> MSHPPSNTPPVKPGGLPLLGHILEFGKNPHAFLMALRHEFGDVAEFRMFHQRMVLLTGSQASEAFYRAPDEVLDQGPAYRIMTPIFGRGVVFDARIERKNQQLQMLMPALRDKPMRTYSEIIVAEVEAMLRDWKDAGTIDLLELTKELTIYTSSHCLLGAEFRHELNTEFAGIYRDLEMGIQPIAYVFP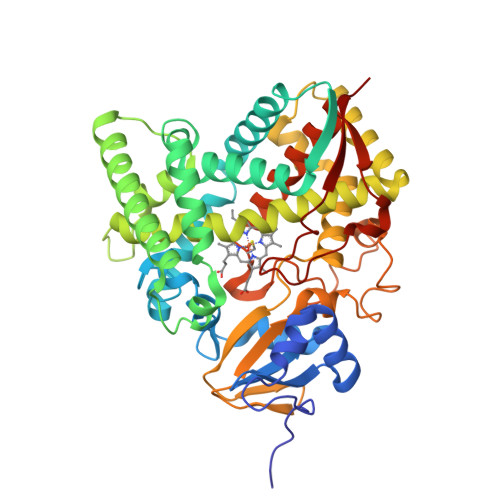NLPLPVFKRRDQARVRLQELVTQIMERRARSQERSTNVFQMLIDASYDDGSKLTPHEITGMLIATIFAGHHTSSGTTAWVLIELLRRPEYLRRVRAEIDALFETHGRVTFESLRQMPQLENVIKEVLRLHPPLILLMRKVMKDFEVQGMRIEAGKFVCAAPSVTHRIPELFPNPELFDPDRYTPERAEDKDLYGWQAFGGGRHKCSGNAFAMFQIKAIVCVLLRNYEFELAAAPESYRDDYRKMVVEPASPCLIRYRRRD>[6x]MDLAKLGLKEVMPTKINLEGLVGDHAFSMEGVGEGNILEGTQEVKISVTKGAPLPFAFDIVSVAFTYGNRAYTGYPEEISDYFLQSFPEGFTYERNIRYQDGGTAIVKSDISLEDGKFIVNVDFKAKDLRRMGPVMQQDIVGMQPSYESMYTNVTSVIGECIIAFKLQTGKHFTYHMRTVYKSKKPVETMPLYHFIQHRLVKTNVDTASGYVVQHETAIAAHSTIKKIEGSLP;>[6x]MTSKVYDPEQRKRMITGPQWWARCKQMNVLDSFINYYDSEKHAENAVIFLHGNATSSYLWRHVVPHIEPVARCIIPDLIGMGKSGKSGNGSYRLLDHYKYLTAWFELLNLPKKIIFVGHDWGAALAFHYAYEHQDRIKAIVHMESVVDVIESWDEWPDIEED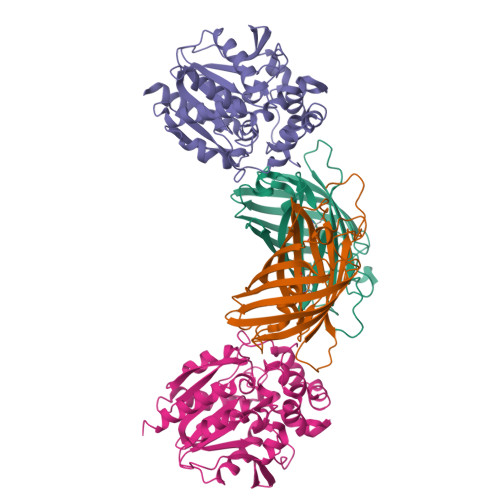IALIKSEEGEKMVLENNFFVETVLPSKIMRKLEPEEFAAYLEPFKEKGEVRRPTLSWPREIPLVKGGKPDVVQIVRNYNAYLRASDDLPKLFIESDPGFFSNAIVEGAKKFPNTEFVKVKGLHFLQEDAPDEMGKYIKSFVERVLKNEQSGLEVLFQ>[2x]SHMSEISRVALFGKLNSLAYKAIEAATVFCKLR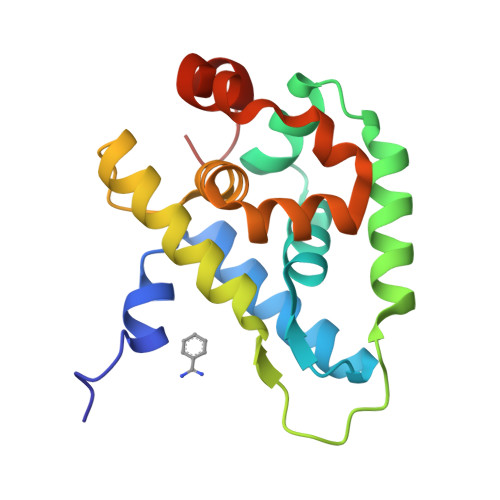GNPYVELVHWFHQILQLPDSDLHQIVRQSGIDPARLAKDLTEALDRLPRGSTSITDLSSHVEEAVERGWVYGSLMFGESQVRTGYLVIGILKTPSLRHALTGLSAEFAKLKVEALTERFDEYVGASPENG> KNIINTSILNLRYESNHLIDLSRYASKINIGSKVNFDPIDKNQIQLFNLESSKIEVILKNAIVYNSMYENFSTSFWIRIPKYFNSISLNNEYTIINCMENNSGWKVS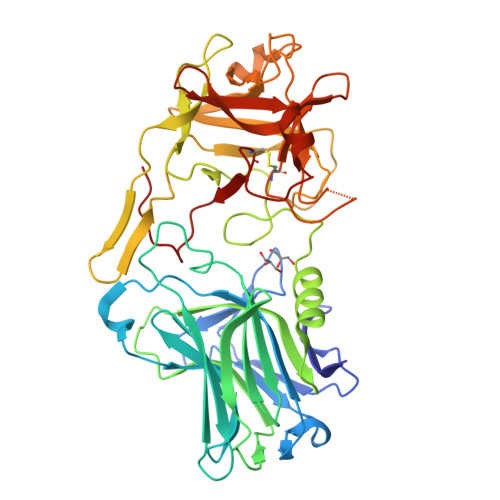LNYGEIIWTLQDTQEIKQRVVFKYSQMINISDYINRWIFVTITNNRLNNSKIYINGRLIDQKPISNLGNIHASNNIMFKLDGCRDTHRYIWIKYFNLFDKELNEKEIKDLYDNQSNSGILKDFWGDYLQYDKPYYMLNLYDPNKYVDVNNVGIRGYMYLKGPRGSVMTTNIYLNSSLYRGTKFIIKKYASGNKDNIVRNNDRVYINVVVKNKEYRLATNASQAGVEKILSALEIPDVGNLSQVVVMKSKNDQGITNKCKMNLQDNNGNDIGFIGFHQFNNIAKLVASNAYNRQIERSSRTLGCSWEFIPVDDGWGERPL>[2x]MQKRAIYPGTFDPITNGHIDIVTRATQMFDHVILAIAASPSKKPMFTLEERVALAQQATAHLGNVEVVGFSDLMANFARNQHATVLIRGLRAVADFEYEMQLAHMNRHLMP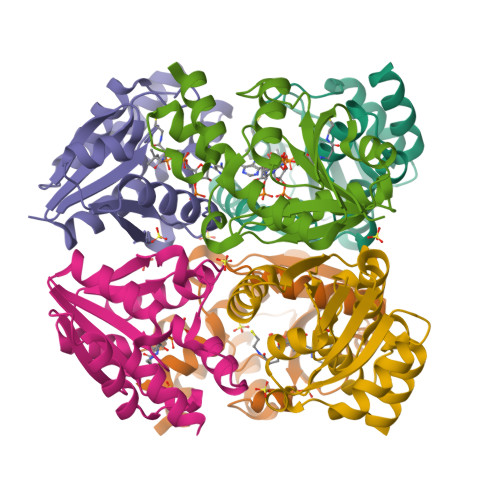ELESVFLMPSKEWSFISSSLVKEVARHQGDVTHFLPENVHQALMAKLA>GSHMESFLLSKVSFVIKKIRLEKGMTQEDLAYKSNLDRTYISGIERNSRNLTIKSLELIMKGLEVSDVVFFEMLIKEILKH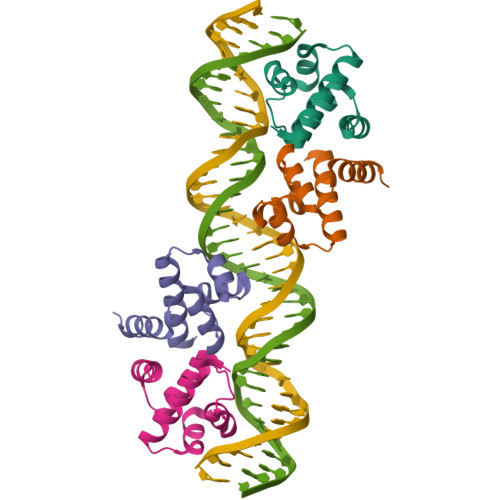D[4x]>MTGSSPALNARQQALLTALNACGDEMSGQQLHRSLDDEASMGLATVYRNLRQLQQRGLVRCRHLPTGEALYAPVDRDRHHLTCVDCGTTQVLDHCPIHGIDVPADSRGDFELLFHTLEFFGFCSSCRPQRSSKP[4x]

SynZur (SYNW2401) is a metallosensor of the Fur family that responds to zinc, and hence a confirmed Zur protein. Using Synechococcus sp. WH8102 as a model we show that its zinc-sensor protein Zur differs from all other known bacterial Zur proteins in overall structure and the location of its sensory zinc site. Thus, Zur in WH8102 regulates both zinc uptake (via znuABC) and storage (via bmtA). Although homologs for the zinc excess sensor SmtB are absent from true marine strains, homologs of the ‘zinc uptake regulator’ Zur were found in every genome inspected, including a range of Synechococcus and Prochlorococcus strains, Trichodesmium erythraeum and Crocosphaera watsonii. These putative bacterial Zur proteins are members of a larger family of metal and peroxide sensors that also comprise Fur (ferric iron uptake regulator), Mur (sensing Mn2+), Nur (sensing Ni2+), Irr (sensing heme) and PerR (sensing peroxide).

The structure was solved to a resolution of 2.1 Å employing single-wavelength anomalous diffraction with fluorescence detected at the zinc K absorption edge (9,666 eV). This approach was necessary because molecular replacement using a range of bacterial Fur-family proteins failed—indicating that SynZur adopts a structure that substantially differs from previously determined structures. The asymmetric unit of the crystal with the space group P65 contains four protein molecules. Interface analysis by PISA36 is consistent with SynZur forming a homodimer, with two dimers present in the asymmetric unit. Each monomer has two zinc ions bound with bond lengths that are within the expected ranges; one is bound tetrahedrally by four Cys residues (83, 86, 123 and 126) and corresponds to the structural site mentioned previously (site 1). Site 1 is located in the DD and tethers the C terminus to a region close to the second zinc site, which is formed by D77, H79, C95 and H115 (site 2). To confirm that this tetrahedral site is involved in zinc sensing, we generated a Cys95Ala mutant protein. However, electrophoretic mobility shift assay (EMSA) experiments demonstrate that the mutant is unable to interact with Zur boxes. Although some Fur-family proteins harbor additional metal-binding sites in an analogous location, SynZur is the first Fur-family protein in which this site is the sole sensory site. Thus, SynZur not only harbors a new zinc-sensing site, but also displays a unique orientation of DD and DBD.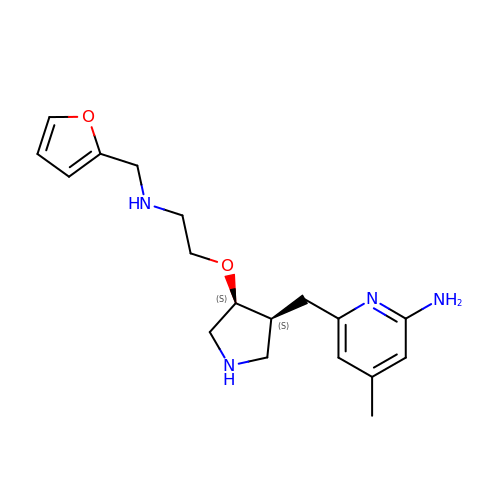6-{[(3S,4S)-4-{2-[(furan-2-ylmethyl)amino]ethoxy}pyrrolidin-3-yl]methyl}-4-methylpyridin-2-amine | C18 H26 N4 O2 | JGPWHIBNRITPFL-WMLDXEAASA-N> RSMETGEVVDCHLSDMLQQLHSVNASKPSERGLVRQEEAEDPACIPIFWVSKWVDYSDKYGLGYQLCDNSVGVLFNDSTRLILYNDGDSLQYIERDGTESYLTVSSHPNSLMKKITLLKYFRNYMSEHLLKAGANITPREGDELARLPYLRTWFRTRSAIILHLSNGSVQINFFQDHTKLILC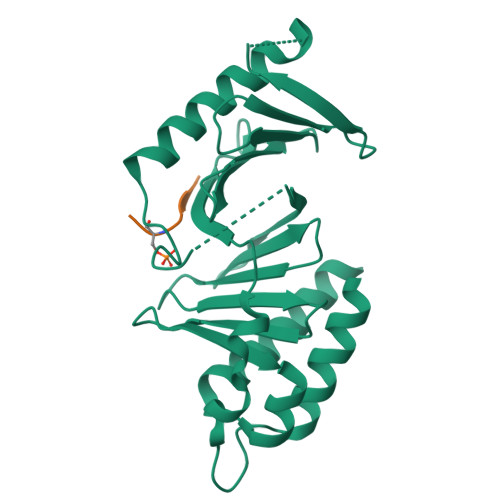PLMAAVTYIDEKRDFRTYRLSLLEEYGCCKELASRLRYARTMVDKLLSSRSASNRLKAS;> ASMWSSM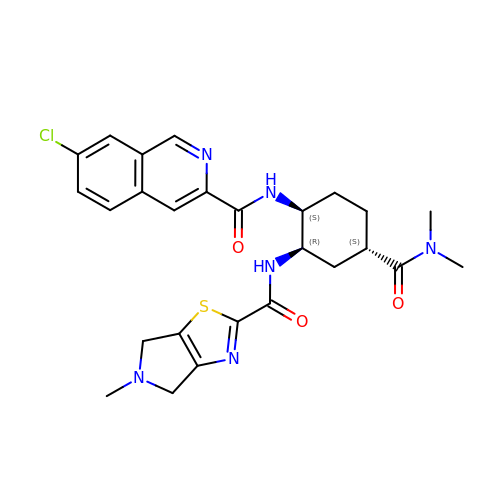7-chloro-N-[(1S,2R,4S)-4-(dimethylcarbamoyl)-2-{[(5-methyl-5,6-dihydro-4H-pyrrolo[3,4-d][1,3]thiazol-2-yl)carbonyl]amino}cyclohexyl]isoquinoline-3-carboxamide | C26 H29 Cl N6 O3 S | GZCKMZURFJCTJE-ZYSHUDEJSA-N>[4x]HHHHHHGSMNLTIIGSGYVGLVTGACLADIGHDVFCLDVDQAKIDILNNGGVPIHEPGLKEVIARNRSAGRLRFSTDIEAAVAHGDVQFIAVGTPPDEDGSADLQYVLAAARNIGRYMTGFKVIVDKSTVPVGTAERVRAAVAEELAKRGGDQMFSVVSNP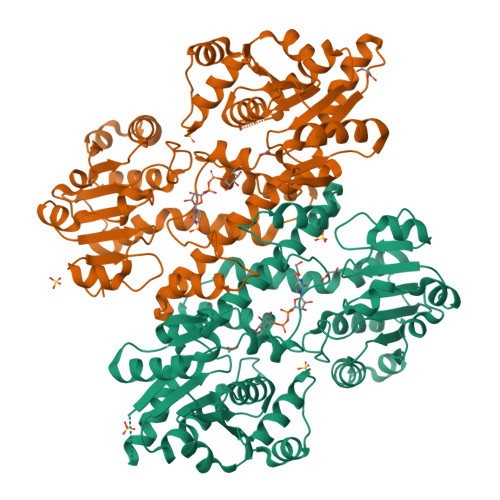EFLKEGAAVDDFTRPDRIVIGCDDDVPGERARELMKKLYAPFNRNHERTLYMDVRSAEFTKYAANAMLATRISFMNELANLADRFGADIEAVRRGIGSDPRIGYHFLYAGCGYGGSCFPKDVEALIRTADEHGQSLQILKAVSSVNATQKRVLADKIVARFGEDLTGRTFAIWGLAFKPNTDDMREAPSRELIAELLSRGARIAAYDPVAQEEARRVIALDLADHPSWLERLSFVDDEAQAARDADALVIVTEWKIFKSPDFVALGRLWKTPVIFDGRNLYEPETMSEQGIEYHPIGRPGSRQAVAARVTGTAPASA2-hydroxy-3-[4-(2-hydroxy-3-sulfopropyl)piperazin-1-yl]propane-1-sulfonic 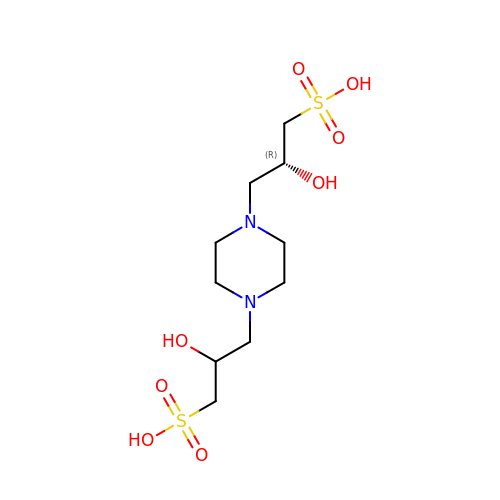acid | C10 H22 N2 O8 S2 | LVQFQZZGTZFUNF-YHMJZVADSA-N>[2x]MSEQTVQVKTTGKILQSPCGPIIHGLEDVLIKSTSISDIDGEKGILWYRGYRIEELARLSTYEEVSYLILYGRLPTKRELEDYINRMKKYRELHPATVEVIRNLAKAHPMFALEAAVAAEGAYDEDNQKLIEALSVGRYKAEEKELAYRIAEKLVAKMPTIVAYHYRFSRGLEVVRPRDDLGHAANFLYMMFGREPDPLA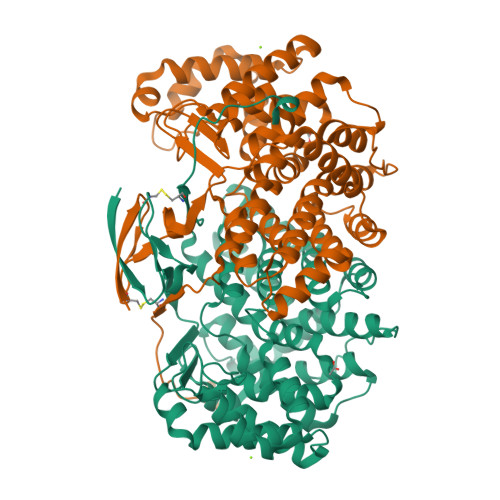SRGIDLYLILHADHEVPASTFAAHVVASTLSDLYSSVAAAIAALKGPLHGGANEMAVRNYLEIGTPAKAKEIVEAATKPGGPKLMGVGHRVYKAYDPRAKIFKEFSRDYVAKFGDPQNLFAIASAIEQEVLSHPYFQQRKLYPNVDFWSGIAFYYMGIPYEYFTPIFAMSRVVGWVAHVLEYWENNRIFRPRACYIGPHDLQYIPLEQR> MSLIIETPSKVILFGEHAVVYGYRAISMAIDLTSTIEI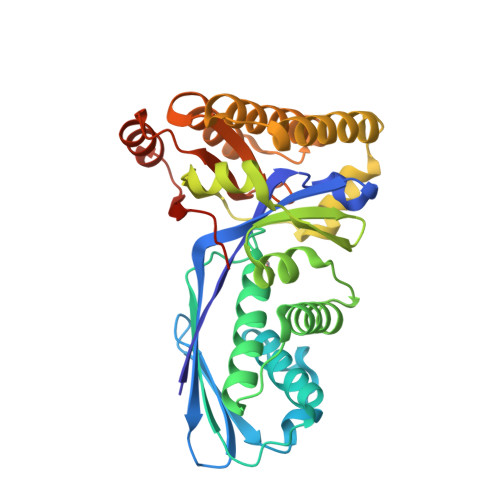KETQEDEIILNLNDLNKSLGLNLNEIKNINPNNFGDFKYCLCAIKNTLDYLNIEPKTGFKINISSKIPISCGLGSSASITIGTIKAVSGFYNKELKDDEIAKLGYMVEKEIQGKASITDTSTITYKGILEIKNNKFRKIKGEFEEFLKNCKFLIVYAEKRKKKTAELVNEVAKIENKDEIFKEIDKVIDEALKIKNKEDFGKLMTKNHELLKKLNISTPKLDRIVDIGNRFGFGAKLTGAGGGGCVIILVNEEKEKELLKELNKEDVRIFNCRMMNEGGSHHHHHH> ETGVFQKAVDQSIEKKIVLRNGTEAFDSWEKPPLPVYTQFYFFNVTNPEEILRGETPRVEEVGPYTYRELRNKANIQFGDNGTTISAVSNKAYVFERDQSVGDPKIDLIRTLNIPVLTVIEWSQVHFLREIIEAMLKAYQQKLFVTHTVDELLWGYKDEILSLIHVFRPDISPYFGLFYEKNGTNDGDYVFLTGEDSYLNFTKIVEWNGKTSLDWWITDKCNMINGTDGDSFHPLITKDEVLYVFPSDFCRSVYITFSDYESVQGLPAFRYKVPAEILANTSDNAGFCIPEGNCLGSGVLNVSICKNGAPIIMSFPHFYQADERFVSAIEGMHPNQEDHETFVDINPLTGIILKAAKRFQINIYVKKLDDFVETGDIRTMVFPVMYLNESVHIDKETASRLKSMINTTGKHHHHHH

Lysosomal integral membrane protein 2 (LIMP-2) is encoded by gene SCARB2, and is also known as scavenger receptor class B member 2 (SCARB2; refs 1, 2). It has N- and C-terminal transmembrane helices (being a type III membrane protein) and a heavily glycosylated 400 residue luminal domain (bearing nine potential N-linked glycosylation sites). The most notable function of LIMP-2 is that it serves as a lysosomal sorting receptor for β-glucocerebrosidase (β-GCase), deficiency of which causes Gaucher disease, a lysosomal storage disease in which glucocerebrosides accumulate. LIMP-2 binds to β-GCase in a pH-dependent manner, and dissociation occurs in acidic late endosomal/lysosomal compartments.

Human LIMP-2 luminal domain containing residues 28–431 was produced by stable expression in HEK293S (GnTI−) cells and crystallized in two space groups, C2221 and C2, at pH 6.5. X-ray diffraction data were collected at the Diamond Light Source, and structures of both crystal forms were determined using the molecular replacement method based on the model of LIMP-2 at lower pH9 and refined at 2.8 Å resolution. The electron density maps for both space groups are of good quality with only 11 terminal residues disordered with 29 and 30 glycosidic units well ordered in the two space groups. The most surprising observation is that we can identify from the well-defined electron density that the sugar attached to N325 is P-Man9GlcNAc2, the first time this sugar, which bears a terminal M6P, has been seen in a protein structure. The D3 arm of the glycan arches over the side chains of H150 and R153 that cap helix α4. The phosphate attached to O6 of the terminal D3 mannose is stabilized in the C2 crystal form by capping the N terminus of helix α5 via hydrogen bonds to the amide groups of R153, E154 and I155. Although our two structures at pH 6.5 are almost identical to each other (root mean squared deviation=0.3 Å for all Cα atoms), they differ significantly from the pH 5.5 structures (root mean squared deviation=0.5–0.6 Å), with the largest difference occurring in the helical bundle of domain II, which includes exactly the region (residues 150–167) identified as the β-GCase binding site. In contrast, at pH 6.5, the helical bundle is very well defined and similar in both space groups. At higher pH, the α4–α5 linker (residues 151–152) folds towards α7, such that α5 tilts about 20° towards α4 and α7, making the bundle more compact and further stabilized by the C-terminal cap of α4 formed by His150 and Arg153. In contrast, H150 caps α4 at higher pH and seems more likely to act as the trigger for the markedly altered conformation of α4 and α5.> MELKHSISDYTEAEFLQLVTTICDAEATS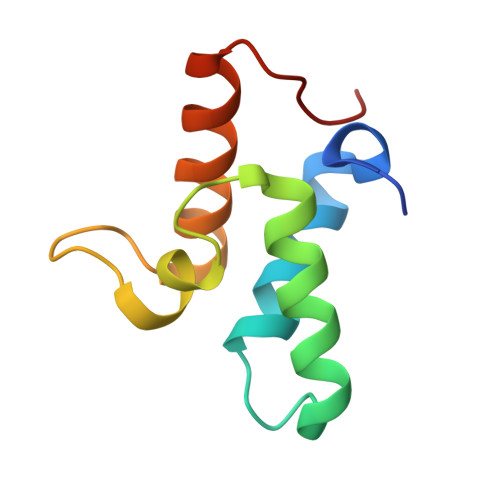EEELDKLITHFEEMTEHPSGSDLIYWPKEGDDDSPSGIVNTVKQWRAANGKSGFKQG> M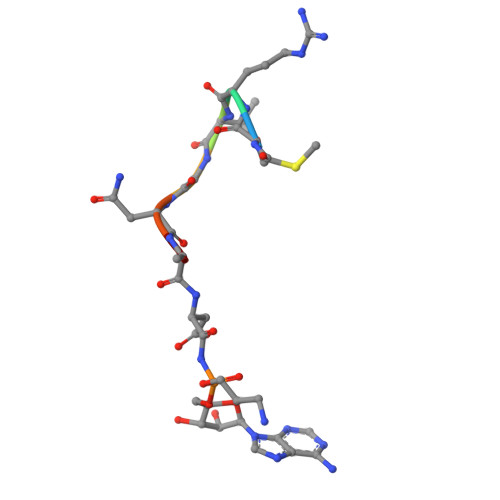RTGNAX(8-oxa-2-azaspiro[4.5]decan-2-yl)(2-{[(pyrazin-2-yl)methyl]amino}pyrimidin-5-yl)methanone | C18 H22 N6 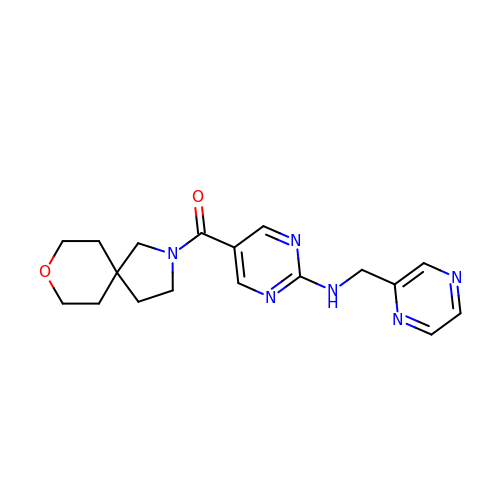O2 | VGRLXWFIXGZRMS-UHFFFAOYSA-N>[2x]GHMDLKTAVFNAARDGKLRLLTKLLASKSKEEVSSLISEKTNGATPLLMAARYGHLDMVEFLLEQCSASIEVGGSVNFDGETIEGAPPLWAASAAGHLKVVQSLLNHGASVNNTTLTNSTPLRAACFDGHLEIVKYLVEHKADLEVSNRHGHTCLMISCYKGHKEIAQYLLEKGADVNRKSVK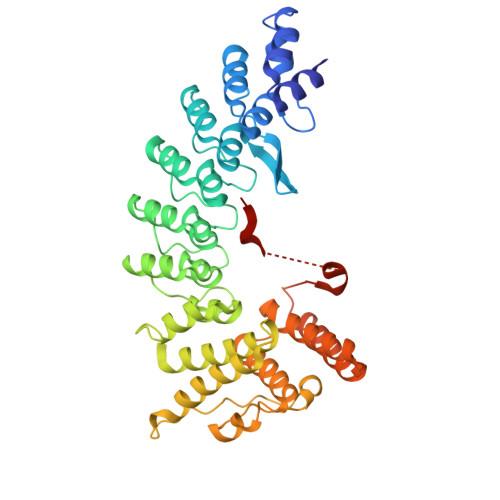GNTALHDCAESGSLDIMKMLLMYCAKMEKDGYGMTPLLSASVTGHTNIVDFLTHHAQTSKTERINALELLGATFVDKKRDLLGALKYWKKAMNMRYSDRTNIISKPVPQTLIMAYDYAKEVNSAEELEGLIADPDEMRMQALLIRERILGPSHPDTSYYIRYRGAVYADSGNFKRCINLWKYALDMQQSNLDPLSPMTASSLLSFAELFGGGSGGGSGGGSGGGSQERGPTWDKNLR> PGSMTLSSNQYQLPLNVRPYTTTWCSQSPSCSNLLAIGHDTGITIYCASEEQTPGSTGLTLQELFTIQTGLPTLHLSFSSSCSYSENLHDGDGNVNSSPVYSLFLACVCQDNTVRLIITKNETIITQHVLGGKSGHHNFVNDIDIADVYSADNRLAEQVIASVGDDCTLIIWRLTDEGPILAGYPLSSPGISVQFRPSNPNQLIVGERNGNIRIFDWTLNLSAEENS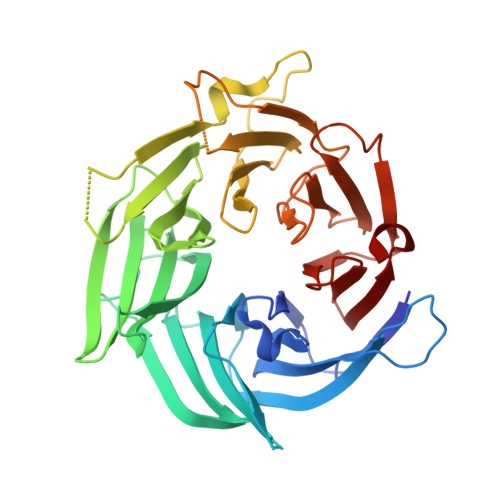QTELVKNPWLLTLNTLPLVNTCHSSGIASSLANVRWIGSDGSGILAMCKSGAWLRWNLFANNDYNEISDSTMKLGPKNLLPNVQGISLFPSLLGACPHPRYMDYFATAHSQHGLIQLINTYEKDSNSIPIQLGMPIVDFCWHQDGSHLAIATEGSVLLTRLMGFTRL>[2x]MAFELPKLPYAFDALEPHFDKETMEIHHDRHHNTYVTKLNAAVEGTDLESKSIEEIVANLDSVPANIQTAV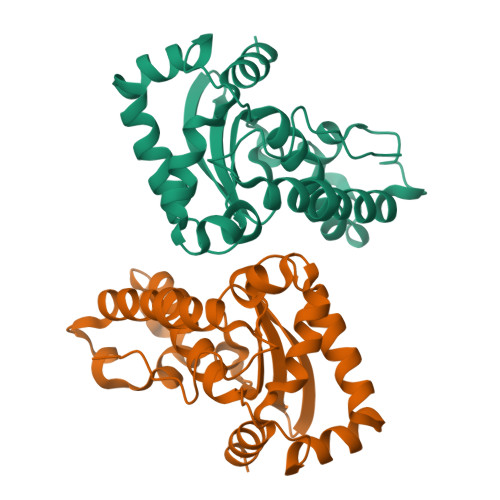RNNGGGHLNHSLFWELLSPNSEEKGTVVEKIKEQWGSLEEFKKEFADKAAARFGSGWAWLVVNNGQLEIVTTPNQDNPLTEGKTPILGLDVWEHAYYLKYQNKRPDYIGAFWNVVNWEKVDELYNATK> GSGPPGPPGPPGPPGAR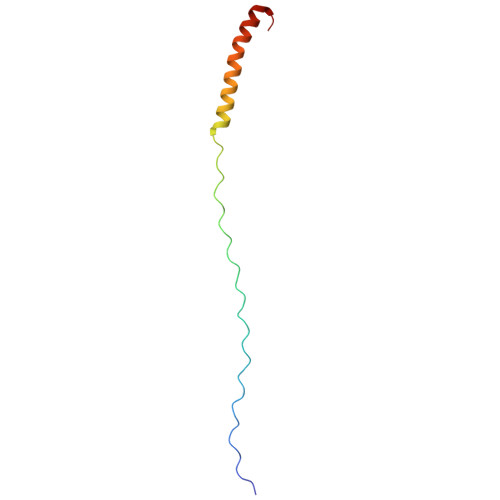GEPGNIGFPGPPGPPGPPGRDATDQHIVDVALKMLQEQLAEVAVSAKREALGAV>KEEFKALKTLSIFYQAGTSKAGNPIFYYVARRFKTGQING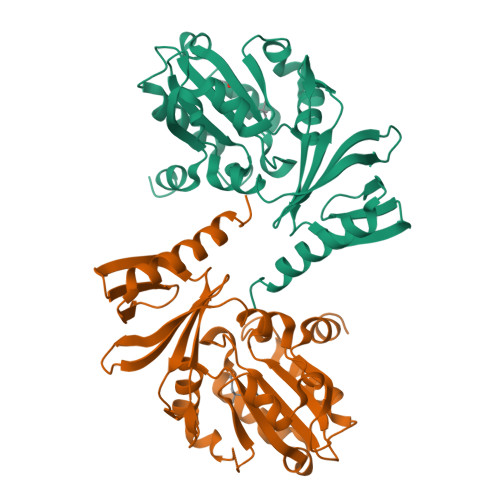DLLIYHVLLTLKPYYAKPYEIVVDLTHTGPSNRFKTDFLSKWFVVFPGFAYDNVSAVYIYNCNSWVREYTKYHERLLTGLKGSKRLVFIDCPGKLAEHIEHEQQKLPAATLALEEDLKVFHNALKLAHKDTKVSIKVGSTAVQVTSAERTKVLGQSVFLNDIYYASEIEEICLVDENQFTLTIANQGTPLTFMHQECEAIVQSIIHIRTRWELSQPD[2x]Streptavidin is a 66-kDa, homotetrameric biotin-binding protein first isolated from the bacterium Streptomyces avidinii. The streptavidin–biotin complex has an equilibrium dissociation constant of 4 × 10–14 M, one of the strongest non-covalent interactions found in nature. The loop connecting β-strands three and four, which is often called “loop 3–4” (residues 45–52), also makes important contributions to biotin binding. When biotin is absent, this loop appears to be highly flexible and dynamically disordered, but it closes upon ligand binding, further burying biotin in the pocket.

The oxidized form of M88 was crystallized in the presence of biotin, yielding well-diffracting crystals belonging to space group P212121 and showing a novel crystal packing arrangement of three tetramers in the asymmetric unit that differs from the packing arrangements seen in previously published structures of streptavidin or mutants. The disulfide bond formed in M88 is also nearly identical in geometry to that predicted by Disulfide by Design 2.0 and that of the natural homolog bradavidin I. The most important difference between the experimentally determined crystal structure and the model is a small rotation of the Cys-49 carbonyl group that moves it away from the newly introduced disulfide bond to resolve a steric clash, but with no major changes to the structure of either loop 3–4 or loop 5–6. In oxidized M88, the backbone hydrogen bond distance between Cys-49 and biotin appears to be very similar to that of Asn-49 in wild-type streptavidin. Additional analysis of the direct binding interactions between biotin and the oxidized form of M88 was performed using the Molegro Molecular Viewer33. This analysis indicates that there are no major changes in biotin binding for the oxidized form of M88 when compared to wild-type streptavidin. M88′s thermostability in the absence of biotin suggests that the disulfide bond promotes the closure of loop 3–4 regardless of the presence of biotin, which promotes interactions between this loop and Trp-120, helping to contribute a substantial amount to the strength of intersubunit interactions. Specifically, Val-47 in the closed conformation of loop 3–4 appears to be in particularly close contact with Trp-120 of loop 7–8 and Leu-25 of loop 1–2, forming a network of hydrophobic interactions that likely provides stabilization to the tetramer.

>MEAGITGTWYNQLGSTFIVTAGADGALTGTYESAVGCAESRYVLTGRYDSAPATDGSGTALGWTVAWKNNYRNCHSATTWSGQYVGGAEARINTQWLLTSGTTEANAWKSTLVGHDTFTKVKPS[12x]> GPDEEPEEPGRRGSFVEMVDNLRGKSGQGYYVEMTVGSPPQTLNILVDTGSSNFAVGAAPHPFLHRYYQRQLSSTYRDLRKGVYVPYTQGKWEGELGTDLVSIPHGPNVTVRANIAAITESDKFFINGSNWEGILGLAYAEIARPDDSLEPFFDSLVKQTHVPNLFSLQLCGAGFPLNQSEVLASVGGSMIIGGIDHSLYTGSLWYTPIRREWYYEVIIVRVEINGQDLKMDCKEYNYDKSIVDSGTTNLRLPKKVFEAAVKSIKAASSTEKFPDGFWLGEQLVCWQAGTTPWNIFPVISLYLMGEVTNQSFRITILPQQYLRPVEDVATSQDDCYKFAISQSSTGTVMGAVIMEGFYVVFDRARKRIGFAVSACHVHDEFRTAAVEGPFVTLD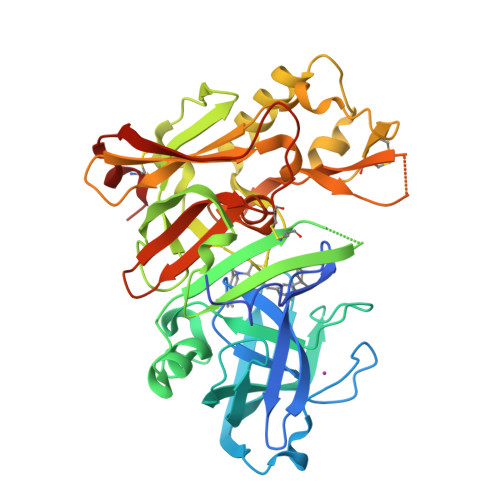MEDCGYNIPQTDES> SLFKDDIQLNEHQVAWYSKDWTAVQSAADSFKEKAENEFFEIIGAINNKTKCSIAQKDYSKFMVENALSQFPECMPAVYAMNLIGSGLSDEAHFNYLMAAVPRGKRYGKWAKLVEDSTEVLIIKLLAKRYQVNTNDAINYKSILTKNGKLPLVLKELKGLVTDDFLKEVTKNV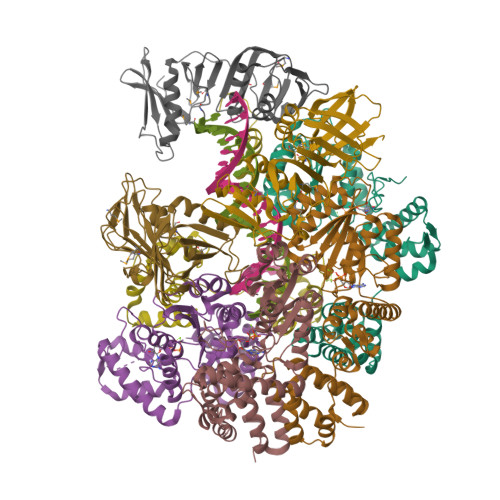KEQKQLKKLALEWGLEHHHHHH;>[4x]GPGGSMITVNEKEHILEQKYRPSTIDECILPAFDKETFKSITSKGKIPHIILHSPSPGTGKTTVAKALCHDVNADMMFVNGSDCKIDFVRGPLTNFASAASFDGRQKVIVIDEFDRSGLAESQRHLRSFMEAYSSNCSIIITANNIDGIIKPLQSRCRVITFGQPTDEDKIEMMKQMIRRLTEICKHEGIAIADMKVVAALVKKNFPDFRKTIGELDSYSSKGVLDAGILSLVTNDRGAIDDVLESLKNKDVKQLRALAPKYAADYSWFVGKLAEEIYSRVTPQSIIRMYEIVGENNQYHGIAANTELHLAYLFIQLACEMQWK;>MKLSKDTTALLKNFATINSGIMLKSGQFIMTRAVNGTTYAEANISDVIDFDVAIYDLNGFLGILSLVNDDAEISQSEDGNIKIADARSTIFWPAADPSTVVAPNKPIPFPVASAVTEIKAEDLQQLLRVSRGLQIDTIAITVKEGKIVINGFNKVEDSALTRVKYSLTLGDYDGENTFNFIINMANMKMQPGNYKLLLWAKGKQGAAKFEGEHANYVVALEADSTHDF[3x]> MTGGMKPPARKPRILNSDGSSNITRLGLEKRGWLDDHYHDLLTVSWPVFITLITGLYLVTNALFALAYLACGDVIENARPGSFTDAFFFSVQTMATIGYGKLIPIGPLANTLVTLEALCGMLGLAVAARLIYARFTRPTAGVLFSSRMVISDFEGKPTLMMRLANLRIEQIIEADVHLVLVRSEISQEGMVFRRFHDLTLTRSRLPIFSLSWTVMHPIDHHSPIYGETDETLRNSHSEFLVLFTGHHEAFAQNVHARHAYSCDEIIWGGHFVDVFTTLPDGRRALDLGKFHEIAQHHHHHH

Recent structural studies of KirBac3.1, an inwardly rectifying potassium (Kir) channel homolog from Magnetospirillum magnetotacticum, have provided important insights into the gating mechanism of eukaryotic Kir channels. These studies, which involved structures of both closed and open states of the channel, identified global conformational changes associated with opening of the lower helix bundle crossing (HBC)4 gate. First, the cytoplasmic domains undergo a rotational movement relative to the plane of the membrane, a conformation termed the “twist state”. Second, interactions that link the second transmembrane domain (TM2) and the slide helix with the cytoplasmic domains (CTDs) are crucial for translating the twist conformation into opening the HBC gate.

To observe the effects of the S205L mutation in the context of an open conformation channel, we therefore created a double mutation (S129R/S205L) in which the HBC gate was engineered to be open and in which the direct consequences of the S205L mutation might be observed by comparison with our previously reported structure of the KirBac3.1 S129R mutation. The mutant channel was therefore crystallized, and the structure was solved to 2.46 Å resolution. The channel crystallized in space group P4212, with one molecule in the asymmetric unit. As a consequence of changes in the loop containing the S205L mutation, there is a change in the rotamer conformation of His177 that leads to a series of changes in the intersubunit interactions at the cytoplasmic interface. By contrast, in the S205L mutant structure, this interaction is replaced by the novel triad His177-Asp197-Arg202. This alternative pairing and charge switching, arising from disruption of the salt bridges centered on His177, lead to a notable charge redistribution, with a rotameric switch in the side chains of Glu173 and Asp175, which now point away from the intersubunit interface and directly into the cytoplasmic pore. Additional electron density was identified within the cytoplasmic cavity consistent with the presence of a potassium ion coordinated by Asp175 and Glu173. We examined the effect of these negatively charged residues on the electrostatic potential of the cytoplasmic pore by comparing the APBS calculations of the S129R mutant and the S129R/S205L double mutant. This analysis revealed a significant decrease in the energetic barrier to potassium permeation in the cytoplasmic pore at the level of Glu173 and Asp175 compared with the KirBac3.1 S129R structure. The results presented here show that the S205L activatory mutation in the CTD stabilizes KirBac3.1 in a novel high-energy open conformation and highlight an important role for the CTD intersubunit interfaces in the control of channel activity.> DLQEDEDGVYFSSYGHYGIHEEMLKDKVRTESYRDFIYQNPHIFKDKVVLDVGCGTGILSMFAAKAGAKKVIAVDQSEILY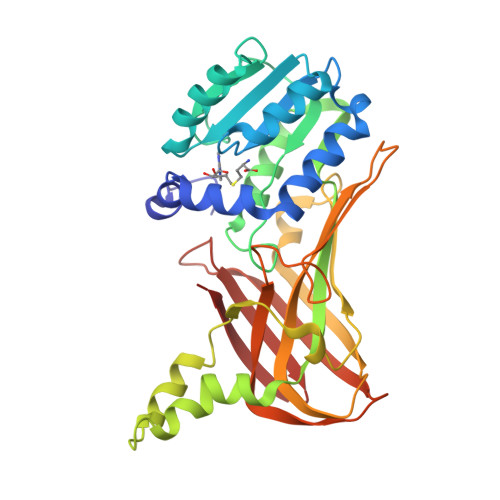QAMDIIRLNKLEDTIVLIKGKIEEVSLPVEKVDVIISEWMGYFLLFESMLDSVLYAKSKYLAKGGSVYPDICTISLVAVSDVSKHADRIAFWDDVYGFNMSCMKKAVIPEAVVEVVDHKTLISDPCDIKHIDCHTTSISDLEFSSDFTLRTTKTAMCTAVAGYFDIYFEKNCHNRVVFSTGPQSTKTHWKQTIFLLEKPFPVKAGEALKGKITVHKNKKDPRSLIVTLTLNSSTQTYSLQ>XFSPAAP[28x];>MSYSGERDNFAPHMALVPMVIEQTSRGERSFDIYSRLLKERVIFLTGQVEDHMANLIVAQMLFLEAENPEKDIYLYINSPGGVITAGMSIYDTMQFIKPDVSTICMGQAASMGAFLL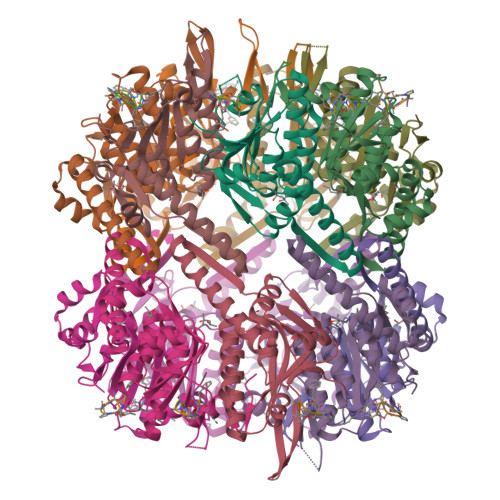TAGAKGKRFCLPNSRVMIHQPLGGYQGQATDIEIHAREILKVKGRMNELMALHTGQSLEQIERDTERDRFLSAPEAVEYGLVDSILTHRN[28x]> MAHHHHHHGTGQDRVVALVDMDCFFVQVEQRQNPHLRNKPCAVVQYKSWKGGGIIAVSYEARAFGVTRSMWADDAKKLCPDLLLAQVRESRGKANLTKYREASVEVMEIMSRFAVIERASIDEAYVDLTSAVQERLQKLQGQPISADLLPSTYIEGLPQGPTTAEETVQKEGMRKQGLFQWLDSLQIDNLTSPDLQLTVGAVIVEEMRAAIERETGFQCSAGISHNKVLAKLACGLNKPNRQTLVSHGSVPQLFSQMPIRKIRSLGGKLGASVIEILGIEYMGELTQFTESQLQSHFGEKNGSWLYAMCRGIEHDPVKPRQLPKTIGCSKNF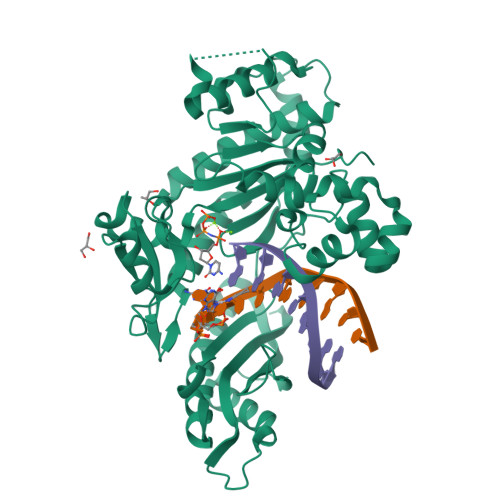PGKTALATREQVQWWLLQLAQELEERLTKDRNDNDRVATQLVVSIRVQGDKRLSSLRRCCALTRYDAHKMSHDAFTVIKNCNTSGIQTEWSPPLTMLFLCATKFSASAPS> MELVKVVFMGWF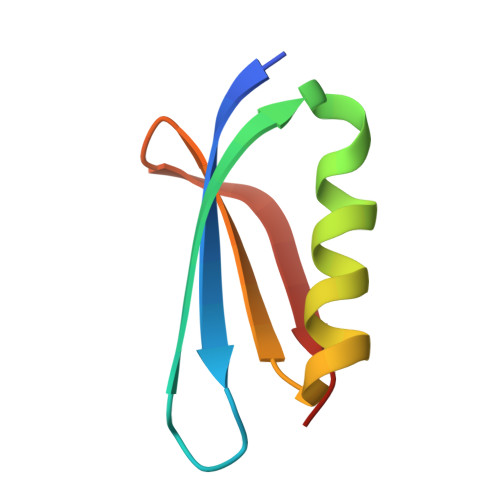KNESMFTKEITMMKDDVQWATTQYAEVNKALVKAFIDDKKVCEVDCRG alpha-D-fucopyranose | C6 H12 O5 | 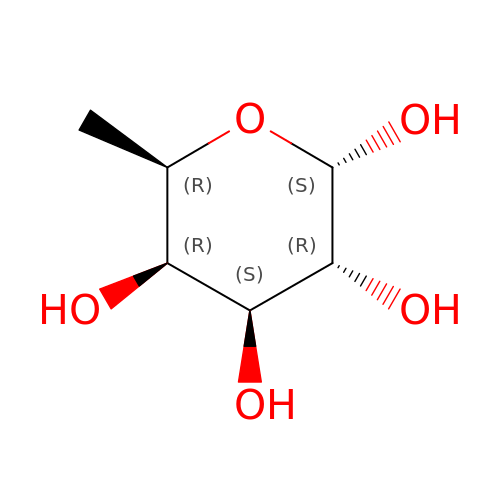SHZGCJCMOBCMKK-PHYPRBDBSA-N>[2x]MSSVIADSQQPAVSEENANKIILDEEKAVIQCNERYKTENDEKGDEETVSWCRKAAKSGNAEAQYLFGMLVYDGRGVQQDNCVAMLWWMKAAEQNHAKALVMLGNLHRKGQCIAENYPKAIAYWKRAAVQNNVWAYHNLGTAYYDGIGVDKNPHEAVRWWKKAAELGFPESQNNLGALYNDGNGVDRDYQEAVFWYRKSALQGDELGQYNLGVAYYYGRG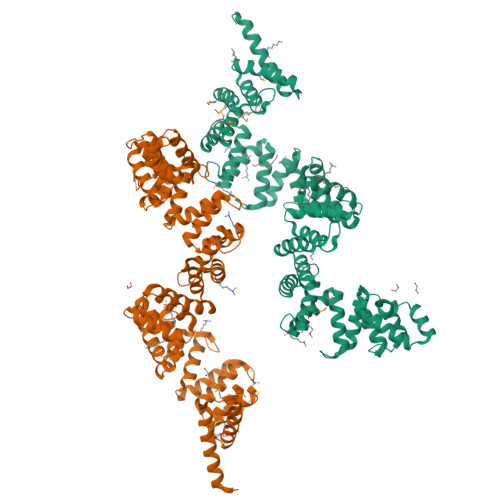IKKDFSEAVSWYKKSAEQDYAQAQHNLGVTYYEGEGIKKDYAKAVYWWKKAAEQGIPQSQYNLGIAYEEGWGAEKNPENAVFWYRKAAEQGHADAQNRLGIAYRYGTGVRKNPALSVKWLEKAAKQGLARAQFNLGKTFYIGAGINKNTDKAVYWFIKAANQGFTEAQAYIGMIYFKGKYVAKNEKKGFYWLKKAAEKDSAKAQAFLGALYIAGNEVKPNIKEGVALTKKAALQGNYEAQTLLGFCYENGLEVKKDLIAAYALYLSASPHFDFAEKARLDLERKLSEQEIAKAISVNTAKLFE>GSMEKAAVNEDGLVIPLIDFSKFLEGDETLKLETAKAILHGFQTAGFIYLKNIPIQPDFREHVFNTSAKFFKLPKEKKLEVGWTTPEANRGYSAPGREKVTQLTDPAEIEKIRSAAPDIKESYEIGREDEPGHPNPWPAEQDDLVGFKSTMNNFFDQCKALHIEVMRAIAVGMGIDANYFDSFVDVGDNILRLLHYPAVKSEVFKINPGQVRAGEHTDYGSITLLFQDSRGGLQVKSPNGQFIDATPIENTVVVNAGDLLARWSNDTIKSTVHRVVEPPKQEDVHPPRYSIAYFCNPNHKSYIEAIPGTYAAESERKYEGINSGK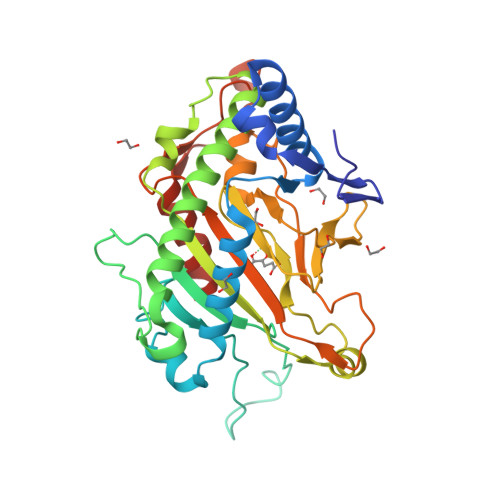YLVQRLAATYLEHHHHHH[4x]> GPGSMMDCDHLLRLGMTAKKILENGKGILAADETPKTLGRRFEKLGITNTEENRRKFREILFSTKGIERYIGGVILNQETFEQTSGSGVPLTELLKKKGIEIGIKLDKGLIDYKEKEKISVGLED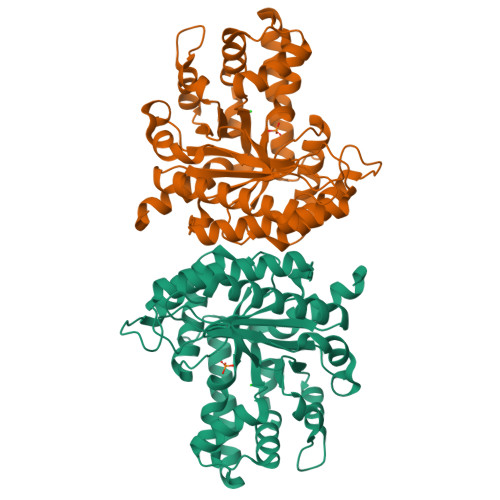LDLRCKSSAFKDATFAKWRSLFYFYDGIPSEDCINENCSILAKYAIICQKNGLVPIVEPEVFLEGDYSMKRSYEVTRQILSTLMKYLNYELVYIPGVLIKASYVTSGQLSNEKYTPKKVATFTLRALLSTIPCGIPGIVFLSGGHGSEDAIGFLNAINMERGCRTWSLSFSFARALTDGVLETWRGDDSNIEEAQKILLETSFKACRGAEGKLWDQE>SNATNNLEKELLDNFKKNITQYAKQLEISIEKVYDEKGSVNAQKDIQNLLSEYANMQEIGEIRFIDKDQIIIATTKQSNRSLINQKANDSSVQKALSLGQSNDHLILKDYGGGKDRVWVYNIPVKVDKKVIGNIYIESKINDVYNQLNNINQ[2x]

Among the 16 TCSs in S. aureus, WalKR (YycGF, VicKR and MicAB) is the only essential TCS involved in diverse cellular processes, including cell wall metabolism, virulence regulation, biofilm production, oxidative stress resistance and antibiotic resistance via direct or indirect regulation of autolysins, the saeRS TCS, haemolysins as well as other key virulence factors13. The sensor kinase of this TCS in S. aureus, WalK, possesses three functional domains including the intracellular kinase, the transmembrane helices as well as the extracellular receptor domain, the first two of which have been found to be conserved across the bacteria that contain this TCS. The other functional domain, the extracellular receptor domain (erWalK) is only present in the bacterial species (for example, Bacillus subtilis, S. aureus, Enterococcus faecalis and Listeria monocytogenes) in which this TCS is essential. Here we report the crystal structure of erWalK, revealing a canonical Per-Arnt-Sim (PAS) domain for signal recognition.

However, the highly anisotropic property of the diffraction data prevented further data processing, which was likely ascribed to the presence of imperfect crystals formed by a mixture of different forms (monomer and dimer) of erWalK6 protein. Further screening of single amino-acid mutants of erWalK6 yielded the construct erWalK6R86M (Arg86 was mutated to Met) that not only exhibited a single peak in size exclusion chromatography analysis (R86M in Supplementary Fig. 1a) but also was crystallized with the crystals diffracting to 1.7 Å resolution. The diffraction data could be processed and the structure was solved by using the seleno-methionine-labelled erWalK6R86M in phase determination. The crystal structure of erWalKR86M revealed that there are two protein molecules in the asymmetric unit that appear to form a tightly packed dimer. The biological relevance of this dimer is unknown; the erWalK686M protein does not form dimer in solution and the dimer is barely found in the wild-type protein when present in high concentrations. Each monomer adopts a canonical PAS domain fold with the presence of five central antiparallel β-strands in a topological order of 2-1-5-4-3. The ends of each monomer are two long helices, directly linking to the transmembrane helices, possibly bridging signal transduction from the extracellular receptor domain to the intracellular kinase domain. The mutation site MSE86 is located in the loop region between the second α-helix and the first β-strand with the side chain of MSE86 facing outwards. Therefore, this mutation is less likely to change the overall structure of the protein, but may contribute to the crystallization. In the ligand-free erWalK conformation, the binding pocket is filled by side chains of E91, R93, V149, Y165 and E167. The salt bridges between E91 and R93, K138 and E167, and the hydrogen bonds between Y165 and E167, Y140 and E167 stabilize the ligand-free conformation.> MGKKQTQRNVFRCNVIGVKNCGKSGVLQALLGRNLMRQKKIREDHKSYYAINTVYVYGQEKYLLL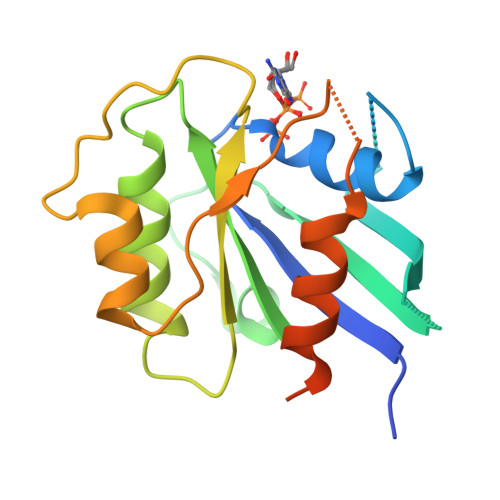HDISESEFLTEAEIICDVVCLVYDVSNPKSFEYCARIFKQHFMDSRIPCLIVAAKSDLHEVKQEYSISPTDFCRKHKMPPPQAFTCNTADAPSKDIFVKLTTMAMYPHVTQADLKSSTFLEHHHHHH> MDAV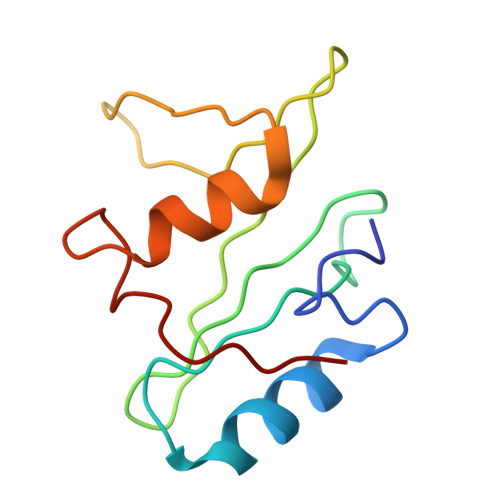AVYHGKISRETGEKLLLATGLDGSYLLRDSESVPGVYCLCVLYHGYIYTYRVSQTETGSWSAETAPGVHKRYFRKIKNLISAFQKPDQGIVIPLQYPVEK1-(4-{2-[(5,6-diphenylfuro[2,3-d]pyrimidin-4-yl)amino]ethyl}phenyl)-3-phenylurea 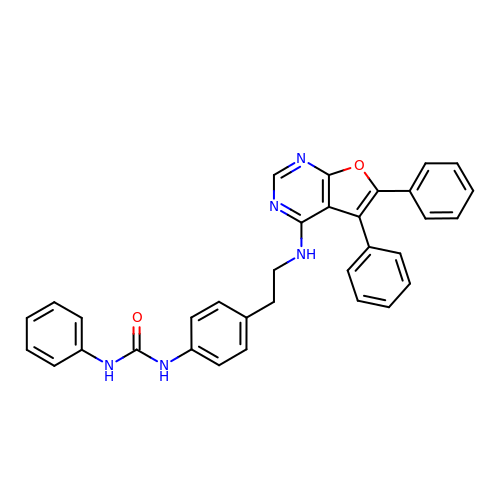| C33 H27 N5 O2 | SPKHBKVYERIGTO-UHFFFAOYSA-N>[2x]MELLKEYNPYLEYRDGELFIEGVSLKELAQTFGTPLYVYSSNFIKERFEAYRKA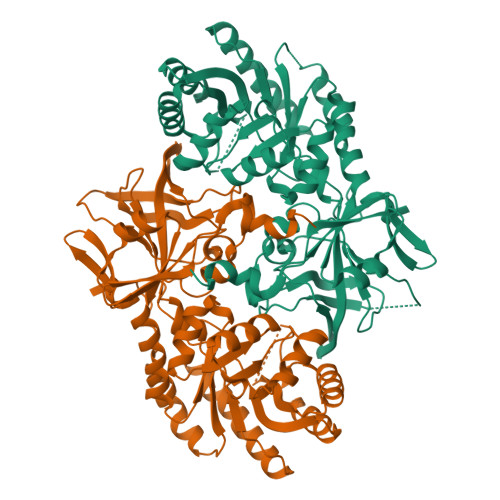FPDALICYAVKANFNPHLVKLLGELGAGADIVSGGELYLAKKAGIPPERIVYAGVGKTEKELTDAVDSEILMFNVESRQELDVLNEIAGKLGKKARIAIRVNPDVDPKTHPYIATGMQKSKFGVDIREAQKEYEYASKLENLEIVGIHCHIGSQILDISPYREAVEKVVSLYESLTQKGFDIKYLDIGGGLGIKYKPEDKEPAPQDLADLLKDLLENVKAKIILEPGRSIMGNAGILITQVQFLKDKGSKHFIIVDAGMNDLIRPSIYNAYHHIIPVETKERKKVVADIVGPICETGDFLALDREIEEVQRGEYLAVLSAGAYGFAMSSHYNMRPRAAEVLVENGSVKLIRKRENYDYIVEPSLDI3,5-DICHLORO-3'-[(DIETHYLAMINO)METHYL]-N-(1,3,5-TRIMETHYL-1H-PYRAZOL-4-YL)BIPHENYL-4-SULFONAMIDE | C23 H28 Cl2 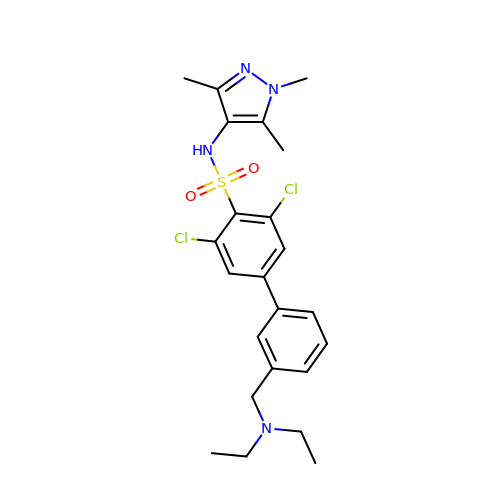N4 O2 S | AGAPYTXFHCVDOQ-UHFFFAOYSA-N>[5x]GVITAGFELKPPPYPLDALEPHMSRETLDYHWGKHHKTYVENLNKQILGTDLDALSLEEVVLLSYNKGNMLPAFNNAAQAWNHEFFWESIQPGGGGKPTGELLRLIERDFGSFEEFLERFKSAAASNFGSGWTWLAYKANRLDVANAVNPLPKEEDKKLVIVKTPNAVNPLVWDYSPLLT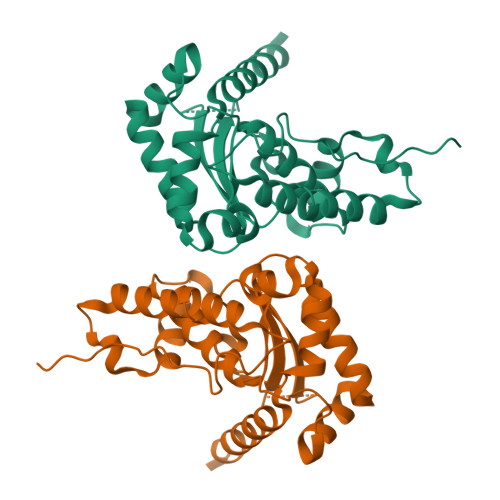IDTWEHAYYLDFENRRAEYINTFMEKLVSWETVSTRLESAIARAVQREQEGTETEDEENPDDEVPEVYLDSDIDVSEVDAAALEHHHHHH Spiroviolene synthase (SvS) from Streptomyces violens was first described by Rabe et al. and represents a bacterial class I diterpene cyclase that we were not able to produce in sufficient quantities for crystallization due to protein instability. Terpene cyclases such as SvS form a variety of complex multicyclic compounds with potent biological activities via carbocationic, electrophilic cyclization cascades of relatively simple substrates, either by metal-ion assisted release of an allylic pyrophosphate (class I mechanism) or by protonation of an oxirane/ene-functionality (class II mechanism). We previously reported a hypothetical ancestor of SvS—SvS-A2 26—which shares 77% sequence identity with the extant enzyme.

To this aim, a small library of 24 variants of SvS-A2 was rationally designed, based on the SvS-A2 crystal structure targeting the active site as well as surrounding residues. The variants could be grouped into four categories based on their substrate preference in a Malachite Green assay: promiscuous (I), inactive (II), diterpene-specific (III), or sesquiterpene-specific (IV). One representative variant of each group was subjected to crystal structure analysis, and Cα rmsd values in the range of 0.35–0.68 Å compared to the parental SvS-A2 structure indicated that none of the variants had significant conformational rearrangements. Therefore, the altered substrate preferences are likely the consequence of steric and/or electronic interactions with substrates, intermediates and/or products, as discussed for the individual variants below. Furthermore, the studied variants were dimeric in the crystal structure and maintained a substantially elevated melting temperature similar to that of SvS-A2. The Gly83Leu substitution may shield off not only Phe79, but also Phe82 and Phe84 from the substrate, which are putatively relevant for cation stabilization. Since our modeling data suggest that Phe84, which is conserved in bacterial sesquiterpene cyclases, is involved in stabilizing cations for both the sesquiterpene and diterpene reactions, sterically blocking this residue by the Gly83Leu exchange results in a near inactive protein.

>MAMTVTEVDLPPIYCPLESAIHPRVHEVEKRAVEWIRRSGMCASEEERAWVIATHSADFFARFAPTAADEDRLLATSLFVYWLFAFDDHRCDNGPLSTRPAQFNALAGRVQRALEAPSAEDNGDRFVPALQDIARRFRSFGTPTQVRRFVHAHRAWLSGVAWQIGNQARGHMPGLDDYLAMRLLSAGGEPTFAMLEIATGAEVPDREMHRPAVRALTEMAIMVAALDNDRHSLRKELSRGHTDQNIYSVLMHHRGMSLQEAVEEATKLRDRILLRFLELHDRVRPGAGAELSTYLQGLRHGIRGNAEWGLRVPRYLSLGRVPDPMEDAPLTWAESPSDSSPSPLPGAPSIAWWWDDALLGA[2x]>MGRLSGKTILVTGAASGIGRAALDLFAREGAS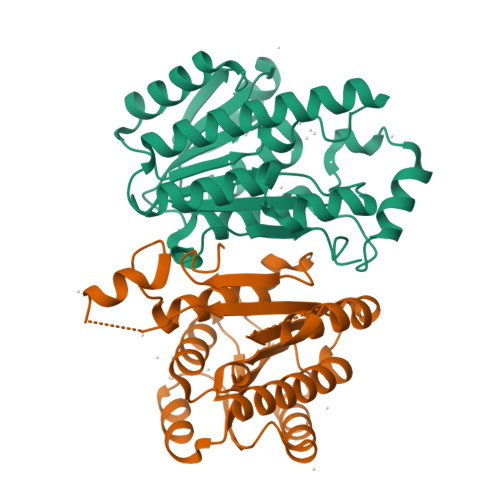LVAVDREERLLAEAVAALEAEAIAVVADVSDPKAVEAVFAEALEEFGRLHGVAHFAGVAHSALSWNLPLEAWEKVLRVNLTGSFLVARKAGEVLEEGGSLVLTGSVAGLGAFGLAHYAAGKLGVVGLARTLALELARKGVRVNVLLPGLIQTPMTAGLPPWAWEQEVGASPLGRAGRPEEVAQAALFLLSEESAYITGQALYVDGGRSIVGPPGLPPGFGPKGGERHAHVL[2x]>[16x]MSTAIVTNVKHFGGMGSALRLSEAGHTVACHDESFKQKDELEAFAETYPQLKPMSEQEPAELIEAVTSAYGQVDVLVSNDIFAPEFQPIDKYAVEDYRGAVEAL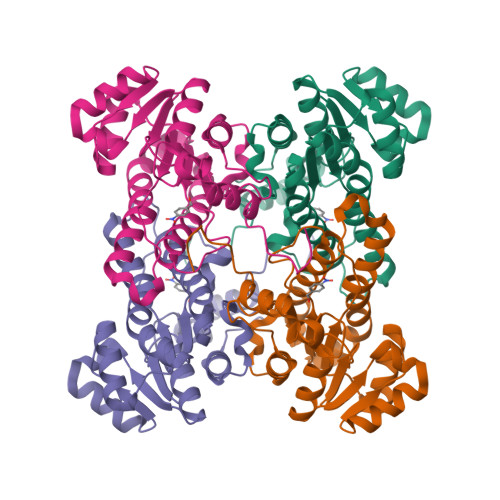QIRPFALVNAVASQMKKRKSGHIIFITSATPFGPWKELSTYTSARAGACTLANALSKELGEYNIPVFAIGPNYLHSEDSPYFYPTEPWKTNPEHVAHVKKVTALQRLGTQKELGELVAFLASGSCDYLTGQVFWLAGGFPMIERWPGMPE>[2x]HMSGPRPVVLSGPSGAGKSTLLKRLLQEHSGIFGFSVSHTTRNPRPGEENGKDYYFVTREVMQRDIAAGD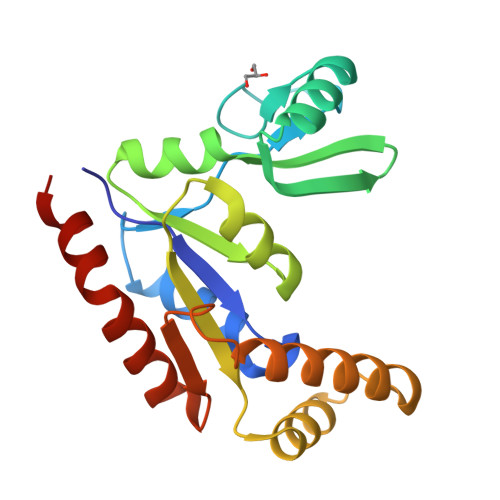FIEHAEFSGNLYGTSKVAVQAVQAMNRICVLDVDLQGVRNIKATDLRPIYISVQPPSLHVLEQRLRQRNTETEESLVKRLAAAQADMESSKEPGLFDVVIINDSLDQAYAELKEALSEEIKKAQRTGA> AMPLDAGGQNSTQMVLAPG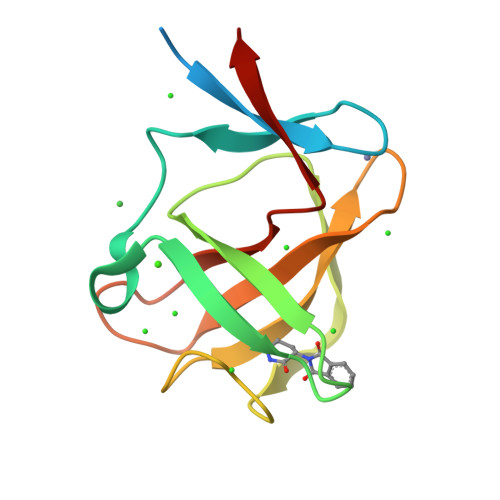ASIFRCRQCGQTISRRDWLLPMGGDHEHVVFNPAGMIFRVWCFSLAQGLRLIGAPSGEFSWFKGYDWTIALCGQCGSHLGWHYEGGSQPQTFFGLIKDRLAEGPAD> ADCPPGWSSYDLYCYQGFNGPQTWDDAERFCTEQAKGGHLVSISDSGEADFVGQLITQNISRPEYYVWTGLRDRRSEQQCNPEWNDGSSIIYTNWDSGESEMCQAFSRWTNFREWMNTNCQQ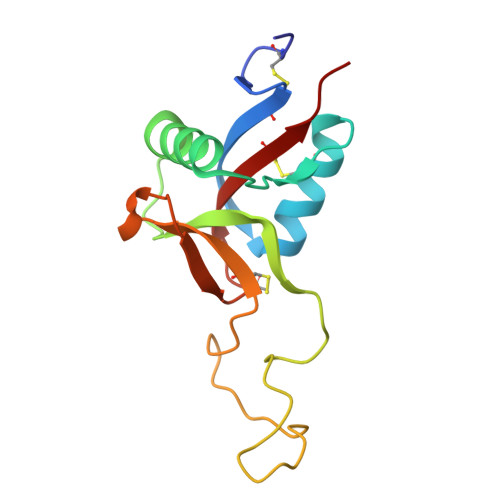KNPFVCKFPPA> MSLTESARIDGVSLYEIVIPMKIPFQISSGTCYTRRSLVVEIREGDLFGYGESAPFEEPFYLGETLETTKVILKNHLLPMILGKEPLSIEEFNHLIKNGIRGNHFARCGVENAYWDLIAKKNKISLKAMIEKKMKNLGVKQEYLASNNYIESGAALGIPEDGRIETLIHQVEESLQEGYRRIKIKIKPGWDVEPLQETRRAVGDHFPLWTDANSSFELDQWETFKAMDAAKCLFHEQPLHYEALLDLKELGERIETPICLDESLISSRVAEFVAKLGISNIWNIKIQRVGGLLEAIKIYKIAT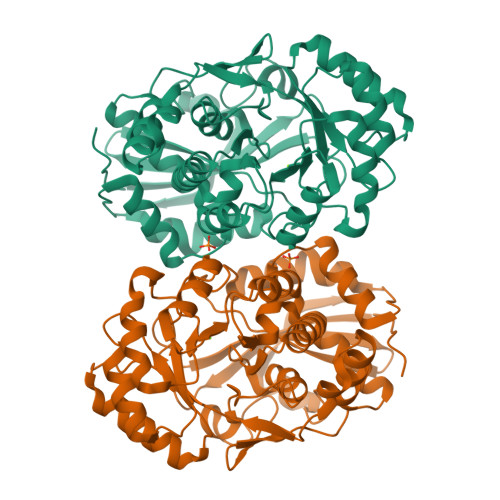DNGIKLWGGTMPESGLGARFLISLASFRGFVFPADVAASEKWYGKGNDLVENTMTDGKIYVPDEPGASFDMTLSHLEALGKKIWESQRGEGHHHHHH> MAHHHHHHHRSDASVIVVGAGPAGLMLAGELRLGGVDVMVLEQLPQRTGESRGLGFTARTMEVFDQRGILPAFGPVETSTQGHFGGRPVDFGVLEGAHYGVKAVPQSTTESVLEEWALGRGAELLRGHTVRALTDEGDHVVVEVEGPDGPRSLTTRYVVGCDGGRSTVRKAAGFDFPGTSASREMFLADIRGCEITPRPIGETVPLGMVMSAP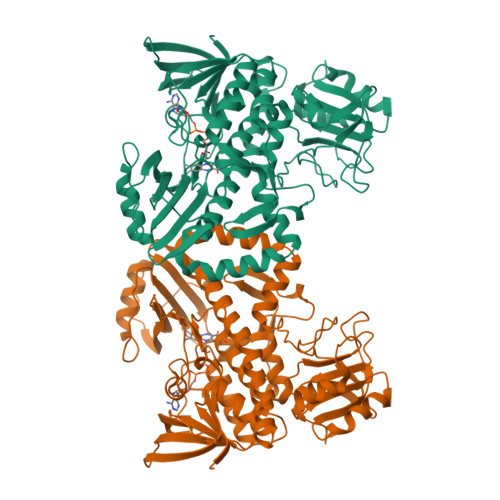LGDGVDRIIVCERGAPARRRTGPPPYQEVAAAWQRLTGQDISHGEPVWVSAFGDPARQVSAYRRGRVLLAGDSAHVHLPAGGQGMNVSVQDSVNLGWKLAAVVSGRAPAGLLDTYHEERHPVGRRLLMNTQAQGMLFLSGDEMQPLRDVLSELIRYDEVSRHLAGMVSGLDIRYEVDGGDHPLLGMRMPHQELVRAHGKTSTTELLHPARGVLLDIADDAEVREAATGWSDRVDIVTASLHDAPPQGPLSDARAVLVRPDGYVAWISPGSRAGLTEALDRWFGPAR> GSMVPPPENVRMNSVNFKNILQWESPAFAKGQLTFTAQYLSYRIFQDKCMQTTLTECDFSSLSKYGDHTLRVRAEFADEHSDWVQITFCPVDDTII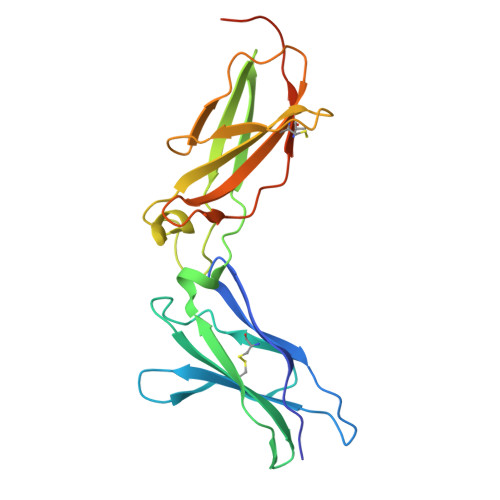GPPGMQVEVLADSLHMRFLAPKIENEYETWTMKNVYNSWTYNVQYWKQGTDEKFQITPQYDFEVLRNLEPWTTYCVQVRGFLPDRNKAGEWSEPVCEQTTHDETVPSAAAHHHHHHHH>HHHHHHLVPRGSMSGADRSPNAG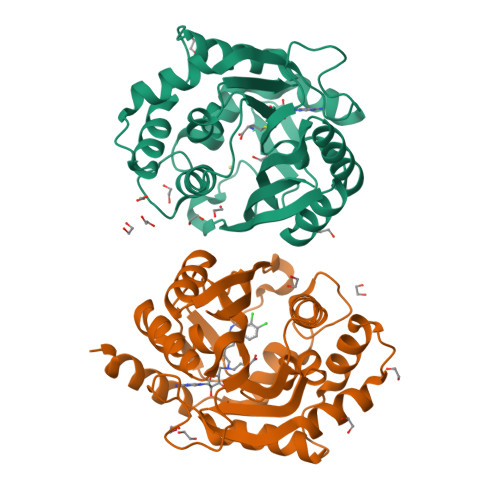AAPDSAPGQAAVASAYQRFEPRAYLRNNYAPPRGDLCNPNGVGPWKLRCLAQTFATGEVSGRTLIDIGSGPTVYQLLSACSHFEDITMTDFLEVNRQELGRWLQEEPGAFNWSMYSQHACLIEGKGECWQDKERQLRARVKRVLPIDVHQPQPLGAGSPAPLPADALVSAFCLEAVSPDLASFQRALDHITTLLRPGGHLLLIGALEESWYLAGEARLTVVPVSEEEVREALVRSGYKVRDLRTYIMPAHLQTGVDDVKGVFFAWAQKVGL[2x]(2~{S})-2-acetamido-~{N}-prop-2-enyl-pentanediamide 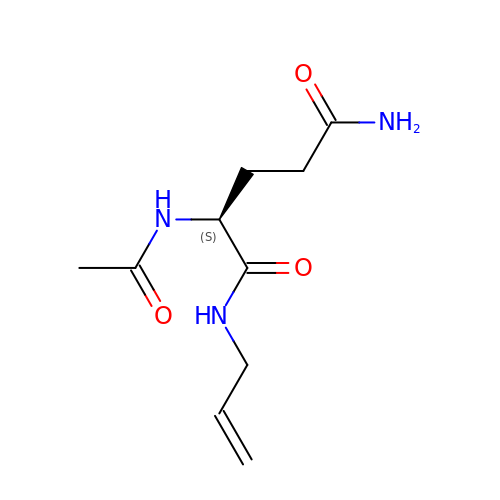| C10 H17 N3 O3 | HRGCJYNJCSFORH-QMMMGPOBSA-N> MPQSRYEKIISARWIITVETDGEVLENHAIAIRDGKIAAIIPAADAAGLEADERLELPDHVLMPGLINLHGHSAMSLLRGLADDKALMDWLTNYIWPTEGKHVHDDFVFDGSLLAMGEMIRGGTTTINDMYFYNAAVARAGLASGMRTFVGCSILEFPTNYASNADDYIAKGMAERSQFLGEDLLTFTLAPHAPYTVSDDTFRKVVTLAEQEDMLIHCHIHETADEVNNSVKEHGQRPLARLQRLGLLSPRLVAAHMVHLNDAEVELAARHGLSTAHNPASNMKLASGISPVSKLMDAGVAVGIGTDGAASNNKLDMLAETRLAALLAKVGTLDPTSVPAAAAIRMATLNGARALGIADKVGSVKVGKQADLIALDLAQLETAP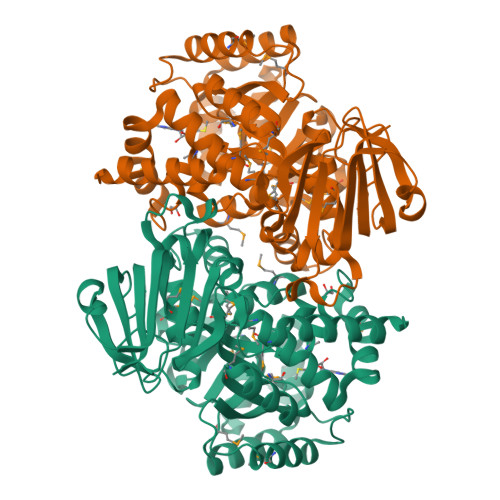AFDPISHVVYAAGREQVSHVWVKGRALMRERKLTTLDESDLKARAGDWRNRILAKEGHHHHHH> GAMAMTEQQKLTFTALQQRLDSLMLRDRLRFSRRLHGVKKVKNPDAQQAIFQEMAKEIDQAAGKVLLREAARPEITYPDNLPVSQKKQDILEAIRDHQVVIVAGETGSGKTTQLPKICMELGRGIKGLIGHTQPRRLAARTVANRIAEELKTEPGGCIGYKVRFSDHVSDNTMVKLMTDGILLAEIQQDRLLMQYDTIIIDEAHERSLNIDFLLGYLKELLPRRPDLKIIITSATIDPERFSRHFNNAPIIEVSGRTYPVEVRYRPIVEEADDTERDQLQAIFDAVDELSQ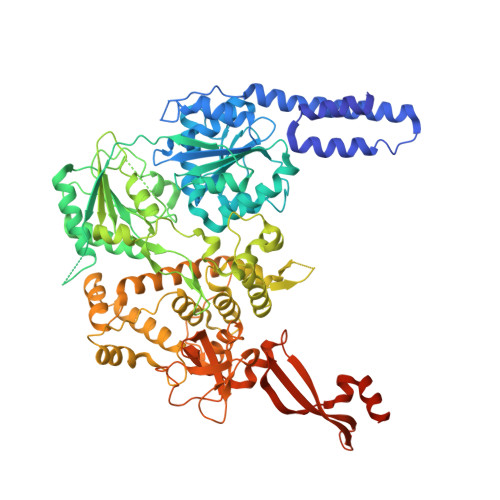ESHGDILIFMSGEREIRATADALNKLNLRHTEILPLYARLSNSEQNRVFQSHSGRRIVLATNVAETSLTVPGIKYVIDPGTARISRYSYRTKVQRLPIEPISQASANQRKGRCGRVSEGICIRLYSEDDFLSRPEFTDPEILRTNLASVILQMTALGLGDIAAFPFVEAPDKRNIQDGVRLLEELGAITTDEQASAYKLTPLGRQLSQLPVDPRLARMVLEAQKHGCVREAMIITSALSIQDPRERPMDKQQASDEKHRRFHDKESDFLAFVNLWNYLGEQQKALSSNAFRRLCRTDYLNYLRVREWQDIYTQLRQVVKELGIPVNSEPAEYREIHIALLTGLLSHIGMKDADKQEYTGARNARFSIFPGSGLFKKPPKWVMVAELVETSRLWGRIAARIDPEWVEPVAQHLIKRTYSEPHWERAQGAVMATEKVTVYGLPIVAARKVNYSQIDPALCRELFIRHALVEGDWQTRHAFFRENLKLRAEVEELEHKS ATP-sensitive potassium channels (KATP) are ion channels that selectively allow potassium ions to permeate the cell. Specifically, they are inhibited by ATP and activated by Mg-ADP. Previous studies have established that the functional KATP channel is a hetero-octamer composed of four inward-rectifying potassium channel 6 (Kir6) subunits and four sulfonylurea receptor (SUR) regulatory subunits. KATP channels in pancreatic islets are composed of Kir6.2 channel subunits and SUR1 regulatory subunits.

During cryo-EM data processing, 3D classification demonstrated continuous conformational heterogeneity of SUR1 in the ATP + GBM state. Specifically, four peripheral SUR1 subunits wobble around the central Kir6.2 channel in small angles. This greatly limited the resolution of the overall cryo-EM density map and deteriorated local map quality of the peripheral SUR1 ABC transporter module. Further improvement of SUR1 map quality at the ATP + GBM state benefited from focused refinement with local search on symmetry-expanded and signal-subtracted particles of the SUR1 ABC-transporter module. The map of “the isolated” SUR1 ABC-transporter module reached a resolution of 4.4 Å and demonstrated markedly enhanced quality, especially for NBDs. Instead, a previously unmodeled density inside the SUR1 central cavity in the ATP + GBM state map has a distinct elongated shape that matches the GBM molecule in an extended conformation. In contrast, this density is not present in the ATP state, where GBM was not supplied into the sample. This unambiguously demonstrates that the extra density inside SUR1 central cavity in the map of the ATP + GBM state represents the GBM molecule. More interestingly, we observed extra density on the degenerate site of SUR1 NBD1. The shape and size of this density matched that of ATPγS. Therefore, we modeled this density as an ATPγS molecule.

> MPLAFCGTENHSAAYRVDQGVLNNGCFVDALNVVPHVFLLFITFPILFIGWGSQSSKVHIHHSTWLHFPGHNLRWILTFILLFVLVCEIAEGILSDGVTESRHLHLYMPAGMAFMAAITSVVYYHNIETSNFPKLLIALLIYWTLAFITKTIKFVKFYDHAIGFSQLRFCLTGLLVILYGMLLLVEVNVIRVRRYIFFKTPREVKPPEDLQDLGVRFLQPFVNLLSKGTYWWMNAFIKTAHKKPIDLRAIGKLPIAMRALTNYQRLCVAFDAQARKDTQSPQGARAIWRALCHAFGRRLILSSTFRILADLLGFAGPLCIFGIVDHLGKENHVFQPKTQFLGVYFVSSQEFLGNAYVLAVLLFLALLLQRTFLQASYYVAIETGINLRGAIQTKIYNKIMHLSTSNLSMGEMTAGQICNLVAIDTNQLMWFFFLCPNLWAMPVQIIVGVILLYYILGVSALIGAAVIILLAPVQYFVATKLSQAQRSTLEHSNERLKQTNEMLRGMKLLKLYAWESIFCSRVEVTRRKEMTSLRAFAVYTSISIFMNTAIPIAAVLITFVGHVSFFKESDLSPSVAFASLSLFHILVTPLFLLSSVVRSTVKALVSVQKLSEFLSSAEIREEQCAPREPAPQGQAGKYQAVPLKVVNRKRPAREEVRDLLGPLQRLAPSMDGDADNFCVQIIGGFFTWTPDGIPTLSNITIRIPRGQLTMIVGQVGCGKSSLLLATLGEMQKVSGAVFWNSNLPDSEGEDPSSPERETAAGSDIRSRGPVAYASQKPWLLNATVEENITFESPFNKQRYKMVIEACSLQPDIDILPHGDQTQIGERGINLSGGQRQRISVARALYQQTNVVFLDDPFSALDVHLSDHLMQAGILELLRDDKRTVVLVTHKLQYLPHADWIIAMKDGTIQREGTLKDFQRSECQLFEHWKTLMNRQDQELEKETVMERKASEPSQGLPRAMSSRDGLLLDEEEEEEEAAESEEDDNLSSVLHQRAKIPWRACTKYLSSAGILLLSLLVFSQLLKHMVLVAIDYWLAKWTDSALVLSPAARNCSLSQECDLDQSVYAMVFTLLCSLGIVLCLVTSVTVEWTGLKVAKRLHRSLLNRIILAPMRFFETTPLGSILNRFSSDCNTIDQHIPSTLECLSRSTLLCVSALTVISYVTPVFLVALLPLAVVCYFIQKYFRVASRDLQQLDDTTQLPLLSHFAETVEGLTTIRAFRYEARFQQKLLEYTDSNNIASLFLTAANRWLEVRMEYIGACVVLIAAATSISNSLHRELSAGLVGLGLTYALMVSNYLNWMVRNLADMEIQLGAVKRIHALLKTEAESYEGLLAPSLIPKNWPDQGKIQIQNLSVRYDSSLKPVLKHVNALISPGQKIGICGRTGSGKSSFSLAFFRMVDMFEGRIIIDGIDIAKLPLHTLRSRLSIILQDPVLFSGTIRFNLDPEKKCSDSTLWEALEIAQLKLVVKALPGGLDAIITEGGENFSQGQRQLFCLARAFVRKTSIFIMDEATASIDMATENILQKVVMTAFADRTVVTIAHRVHTILSADLVMVLKRGAILEFDKPETLLSQKDSVFASFVRADK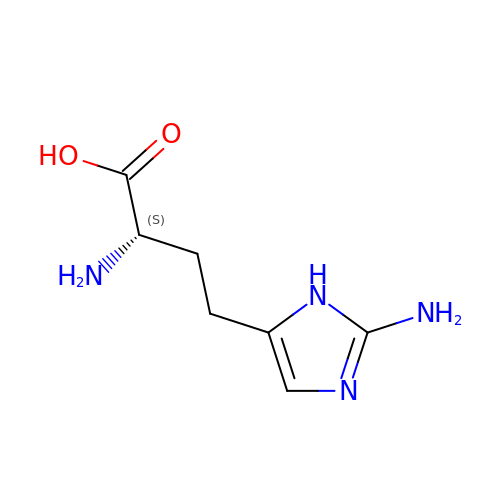(2S)-2-amino-4-(2-amino-1H-imidazol-5-yl)butanoic acid | C7 H12 N4 O2 | FXIIKDXCDODGRI-YFKPBYRVSA-N> MRVRTLDDNGDWTFGRGKADYITSKKAIAQTVSTRIKSWANDNPLAMNANIDWKDLLGRKGTEDTILREIERVVVQTDGVIRVTELEVIKTE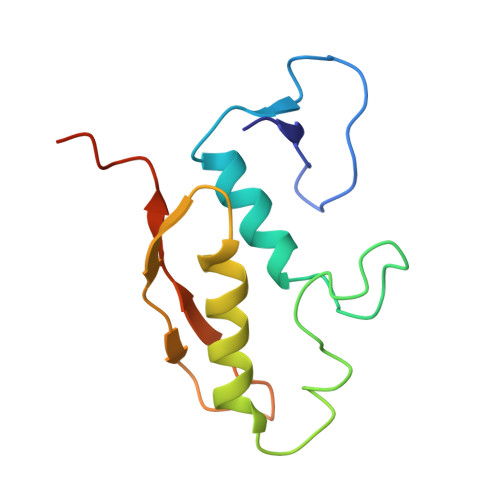KRVQSILLSYDTIYDDSETLEINDL> DNQFYSVEVGDSTFTVLKRYQNLKPIGSGAQGIVCAAYDAVLDRNVAIKKLSRPFQNQTHAKRAYRELVLMKCVNHKNIISLLNVFTPQKTLEEFQDVYLVMELMDANLCQVIQMELDHERMSYLLYQMLCGIKHLHSAGIIHRDLKPSNIVVKSDCTLKILDFGLARTAGTSFMMTPYVVTRYYRAPEVILGMGYKENVDIWSVGCIMGEMVRHKILFPGRDYIDQWNKVIEQLGTPCPEFMKKLQPTVRNYVENRPKYAGLTFPKLFPDSLFPADSEHNK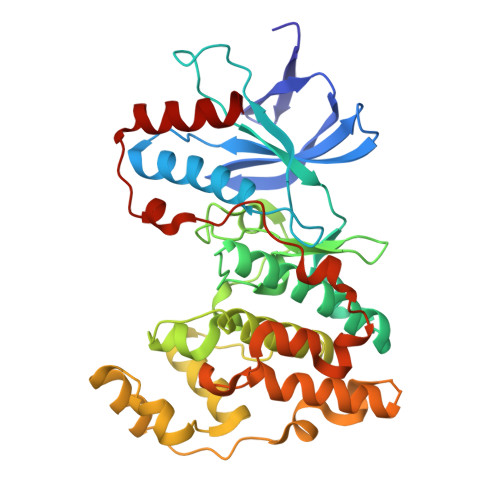LKASQARDLLSKMLVIDPAKRISVDDALQHPYINVWYDPAEVEAPPPQIYDKQLDEREHTIEEWKELIYKEVMN> RNLMIVDGTNLGFRFKHNNSKKPFASSYVSTIQSLAKSYSARTTIVLGDKGKSVFRLEHLP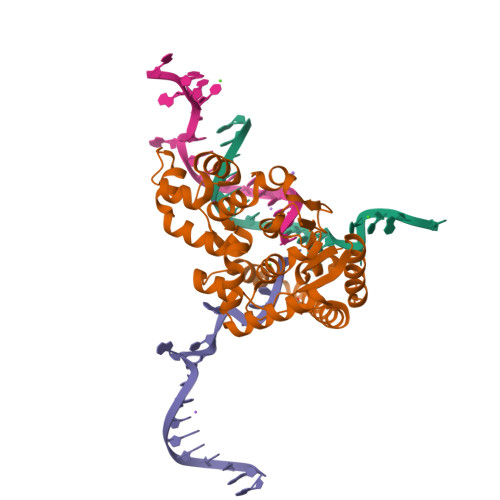EYKGNRDEKYAQRTEEEKALDEQFFEYLKDAFELCKTTFPTFTIRGVEADDMAAYIVKLIGHLYDHVWLISTDGKWDTLLTDKVSRFSFTTRREYHLRDMYEHHNVDDVEQFISLKAIMGDLGDNIRGVEGIGAKRGYNIIREFGNVLDIIDQLPLPGKQKYIQNLNASEELLFRNLILVDLPTYCVDAIAAVGQDVLDKFTKDILEIAEQ>MAGDTTITIVGNLTADPELRFTPSGAAVANFTVASTPRIYDRQTGEWKDGEALFLRCNIWREAAENVAESLTRGARVIVSGRLKQ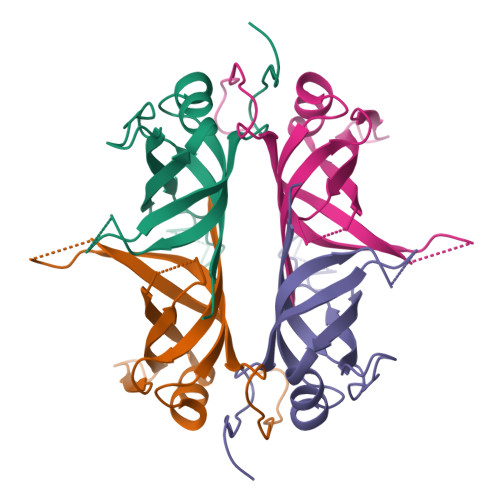RSFETREGEKRTVIEVEVDEIGPSLRYATAKVNKASRSGGFGSGSRPAPAQTSSASGDDPWGSAPASGSFGGGDDEPPF[4x]> GS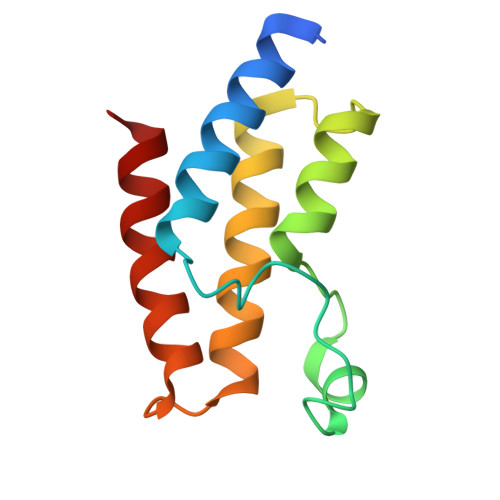AENESTPIQQLLEHFLRQLQRKDPHGFFAFPVTDAIAPGYSMIIKHPMDFGTMKDKIVANEYKSVTEFKADFKLMCDNAMTYNRPDTVYYKLAKKILHAGFKMMSK> GGEPAWDSPLRRVLAELNRIPSSRRRAARLFEWLIAPMPPDHFYRRLWEREAVLVRRQDHTYYQGLFSTADLDSMLRNEEVQFGQHLDAARYINGRRETLNPPGRALPAAAWSLYQAGCSLRLLCPQAFSTTVWQFLAVLQEQFGSMAGSNVYLTPPNSQGFAPHYDDIEAFVLQLEGRKLWRVYRPRVPTEELALTSSPNFSQDDLGEPVLQTVLEPGDLLYFPRGFIHQAECQDGVHSLHLTLSTYQRNTWGDFLEAILPLAVQAAMEENVEFRRGLPRDFMDYMGAQHSDSKDPRRTAFMEKVRVLVARLGHFAPVDAVADQRAKDFIHDSLPP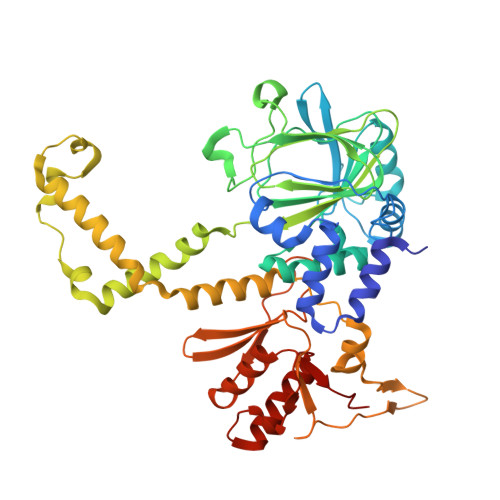VLTDRERALSVYGLPIRWEAGEPVNVGAQLTTETEVHMLQDGIARLVGEGGHLFLYYTVENSRVYHLEEPKCLEIYPQQADAMELLLGSYPEFVRVGDLPCDSVEDQLSLATTLYDKGLLLTKMPLALN> IFNGRPAQKGTTPWIAMLSHLNGQPFCGGSLLGSSWIVTAAHCLHQSLDPKDPTLRDSDLLSPSDFKIILGKHWRLRSDENEQHLGVKHTTLHPQYDP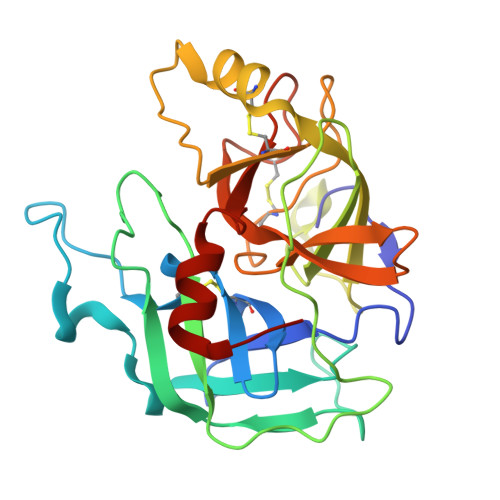NTFENDVALVELLESPVLNAFVMPICLPEGPQQEGAMVIVSGWGKQFLQRFPETLMEIEIPIVDHSTCQKAYAPLKKKVTRDMICAGEKEGGKDACAGDSGGPMVTLNRERGQWYLVGTVSWGDDCGKKDRYGVYSYIHHNKDWIQRVTGVRN6,7-dimethoxy-2-methyl-~{N}-[(1~{R})-1-phenylethyl]quinazolin-4-amine | C19 H21 N3 O2 | 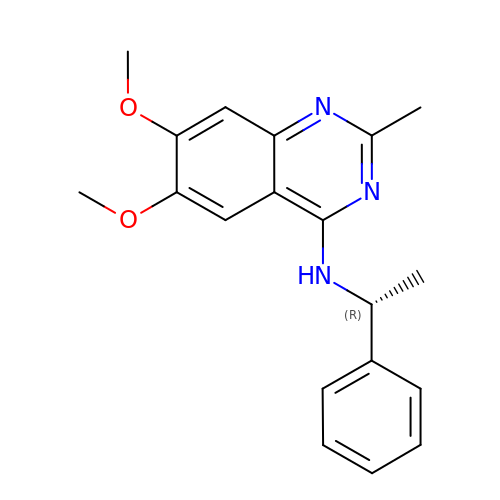SQSDNOVLVOTMJE-GFCCVEGCSA-N> SGISLDNSYKMDYPEMGLCIIINNKNFHKSTGMTSRSGTDVDAANLRETFRNLKYEVRNKNDLTREEIVELMRDVSKEDHSKRSSFVCVLLSHGEEGIIFGTNGPVDLKKITNFFRGDRCRSLTGKPKLFIIQACRGTELDCGIETDSGVDDDMACHKIPVAADFLYAYSTAPGYYSWRNSKDGS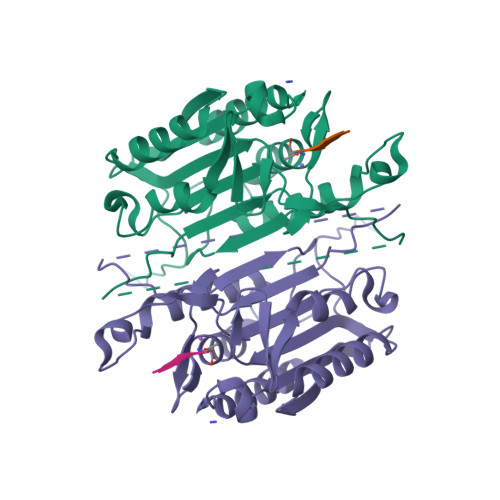WFIQSLCAMLKQYADKLEFMHILTRVNRKVATEFESFSFDATFHAKKQIPCIVSMLTKELYFYHH>MRKIVLPGDLLSTNPRAAGYGTYVEGGKVYAKIIGLFDQTETHVRVIPLKGRYTPSVGDVVIGIIREVAANGWAVDIYSPYQAFLPVSENPEMKPNKKPNEVLDIGDAIIAKVLNIDPKMKVTLTMKDRICRPIRFGRIVAINPARVPRVIGKKGSMIKLLKSELDVQIVVGQNGLIWVNGDRRKVSIAEEAIYLIEQEAHTEGLTDRVAEFIKRRKADVGIQHHHHHH[3x];>[3x]MSEFNEKPEKLIVDGLRLDGRKFDELR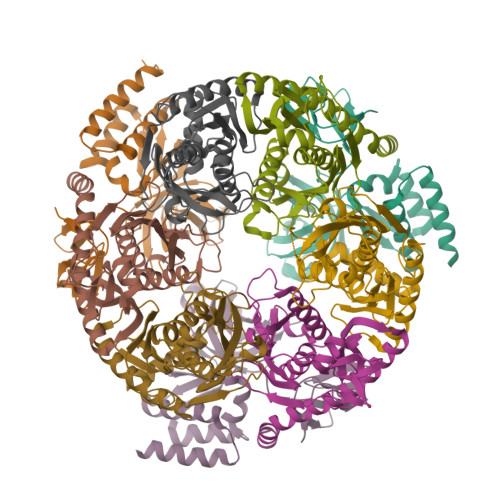PIKIEASVLKRADGSCYLEMGKNKVIAAVFGPREVHPRHLQDPSKAIIRYRYNMAPFSVEERKRPGPDRRSIEISKVSKEAFEAVIMKELFPRSAIDIFVEVLQADAGSRTACLNAASVALVDAGVPMKGMITSVAVGKADGQLVLDPMKEEDNFGEADMPFAFLIRNGKIESIALLQMDGRMTRDEVKQAIELAKKGALQIYEMQREAILRRYIEVGEEMDEITEGGEDA;>[3x]MPEDILVDIKRDYVLSKLRDNERIDGRGFDEFRKVEIIPNVIEKAEGSALVKLGDTQVVVGVKMQPGEPYPDTPDRGVIIVNAELVPLASPTFEPGPPDENSIELARVVDRGIRESEAVDLSKLVIEEGEKVWIVFVDIHALDDDGNLLDASALAAIAALMNTKVPAERFDLGEDYLLPVRDLPVSVTSLIVGNKYLVDPSREEMSVGDTTLTITTDKDDNVVAMQKSGGYLLDEKLFDELLDVSINCARKLREKFKEI>HEDEIKKLRTSGSMTQNPHEVARVRNLNRIIMGKYEIEPWYFSPYPIELTDEDFIYIDDFTLQYFGSKKQYERYRKKCTLRHPPGNEIYRDDYVSFFEIDGRKQRTWCRNLCLLSKLFLDHKTLYYDVDPFLFYCMTRRDELGHHLVGYFSKEKESADGYNVACILTLPQYQRMGYGKLLIEFSYELSKKENKVGSPQKPLSDLGLLSYRAYWSDTLITLLVEHQKEITIDEISSMTSMTTTDILHTAKTLNILRYYKGQHIIFLNEDILDRYNRLKAKKRRTIDPNRLIWKPPVFTASQLRFAW[3x];>[3x]MTDELKSYEALKAELKKSLQDRREQEDTFDNLQQEIYDKETEYFSHNSNNNHSGHGGAHGSKSHYSGNIIKGFDTFSKSHHSHADSAFNNNDRIFSLSSATYVKQQHGQSQND;>[3x]SSNSRFRHRKISVKQHLKIYLPNDLKHLDKDELQQREVVEIETGVEKNEEKEVHLHRILQMGSGHTKHKDYIPTPDASMTWNEYDKFYTGSFQETTSYIKFSATVEDCCGTNYNMDERDETFLNEQVNKGSSDILTEDEFEILCSSFEHAIHERQPFLSMDPESILSFEELKPTLIKSDMADFNLRNQLNHEINSHKTHFITQFDPVSQMNTRPLIQLIEKFGSKIYDYWRERKIEVNGYEIFPQLKFERPGEKEEIDPYVCFRRREVRHPRKTRRIDILNSQRLRALHQELKNAKDLALLVAKRENVSLNWINDELKIFDQRVKIKNLKRSLNISGEDDDLINHKRKRPT;>[3x]MDPSLVLEQTIQDVSNLPSEFRYLLEEIGSNDLKLIEEKKKYEQKESQIHKF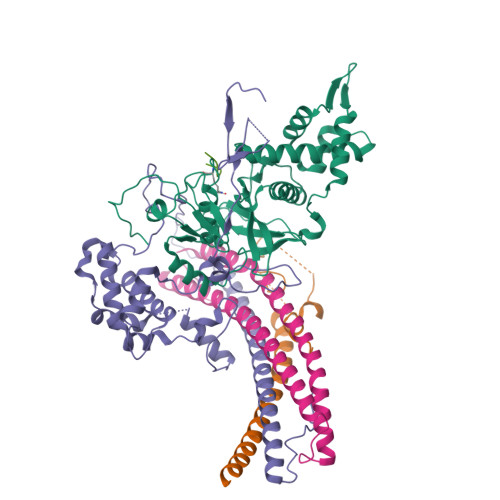IRQQGSIPKHPQEDGLDKEIKESLLKCQSLQREKCVLANTALFLIARHLNKLEKNIALLEEDGVLAPV;>SGAKDSGSLR[3x]>LKFSPQLLSLLSLKTSLSGPPSAFQDWKVPVNGQNDAVWCSWSGVVCDNVTAQVISLDLSHRNLSGRIPIQIRYLSSLLYLNLSGNSLEGSFPTSIFDLTKLTTLDISRNSFDSSFPPGISKLKFLKVFNAFSNNFEGLLPSDVSRLRFLEELNFGGSYFEGEIPAAYGGLQRL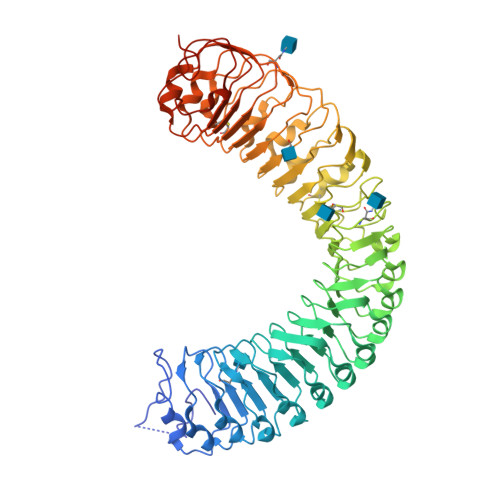KFIHLAGNVLGGKLPPRLGLLTELQHMEIGYNHFNGNIPSEFALLSNLKYFDVSNCSLSGSLPQELGNLSNLETLFLFQNGFTGEIPESYSNLKSLKLLDFSSNQLSGSIPSGFSTLKNLTWLSLISNNLSGEVPEGIGELPELTTLFLWNNNFTGVLPHKLGSNGKLETMDVSNNSFTGTIPSSLCHGNKLYKLILFSNMFEGELPKSLTRCESLWRFRSQNNRLNGTIPIGFGSLRNLTFVDLSNNRFTDQIPADFATAPVLQYLNLSTNFFHRKLPENIWKAPNLQIFSASFSNLIGEIPNYVGCKSFYRIELQGNSLNGTIPWDIGHCEKLLCLNLSQNHLNGIIPWEISTLPSIADVDLSHNLLTGTIPSDFGSSKTITTFNVSYNQLIGPIPSGSFAHLNPSFFSSNEGLCGDLVGKPCNSDRFNAGNADIDG[2x]> MSGFDLSEVAGPVAEVIDDKNEEVEFVVFGVQTQPNKLVVDAKGKGGLEEVKAALKEDALQFAYYRTISGDEESKRVKFVFISWAGEGIKKPKLRAVMSILKGDVKNVINNFHIE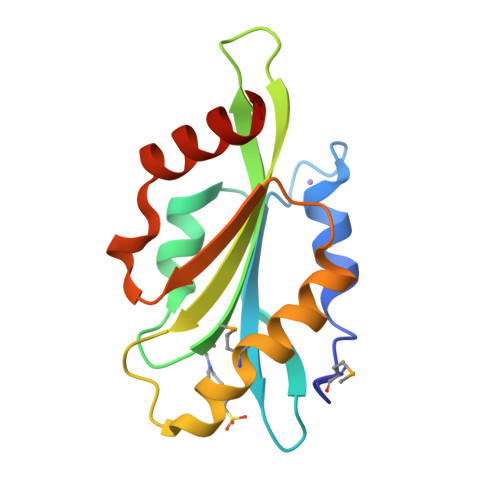LHATSLDDLVEDEIAAKIKLEHHAHHH>TKTKIMGILNVTPDSFSDGGKFNNVESAVTRVKAMMDEGADIIDVGGVSTRPGHEMITVEEELNRVLPVVEAIVGFDVKISVDTFRSEVAEACLKLGVDIINDQWAGLYDHRMFQVVAKYDAEIVLMHNGNGNRDEPVVEEMLTSLLAQAHQAKIAGIPSNKIWLDPGIGFAKTRNEEAEVMARLDELVATEYPVLLATSRKRFTKEMMGYDTTPVERDEVTAATTAYGIMKGVRAVRVHNVELNAKLAKGIDFLK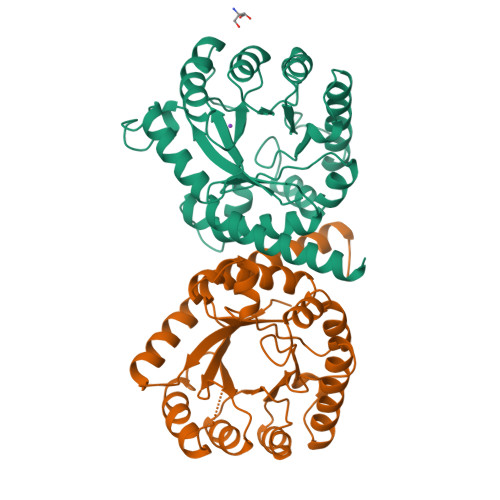ENENARHNFS[2x]>[2x]MWELTILHTNDVHSRLEQTSEDSSKCVNASRCMGGVARLFTKVQQI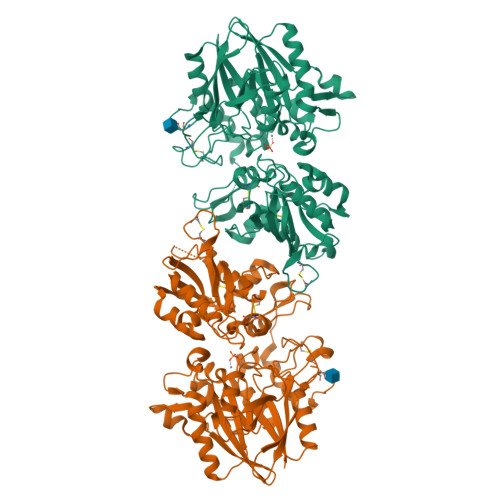RRAEPNVLLLDAGDQYQGTIWFTVYKGAEVAHFMNALRYDAMALGNHEFDNGVEGLIEPLLKEAKFPILSANIKAKGPLASQISGLYLPYKVLPVGDEVVGIVGYTSKETPFLSNPGTNLVFEDEITALQPEVDKLKTLNVNKIIALGHSGFEMDKLIAQKVRGVDVVVGGHSNTFLYTGNPPSKEVPAGKYPFIVTSDDGRKVPVVQAYAFGKYLGYLKIEFDERGNVISSHGNPILLNSSIPEDPSIKADINKWRIKLDNYSTQELGKTIVYLDGSSQSCRFRECNMGNLICDAMINNNLRHTDEMFWNHVSMCILNGGGIRSPIDERNNGTITWENLAAVLPFGGTFDLVQLKGSTLKKAFEHSVHRYGQSTGEFLQVGGIHVVYDLSRKPGDRVVKLDVLCTKCRVPSYDPLKMDEVYKVILPNFLANGGDGFQMIKDELLRHDSGDQDINVVSTYISKMKVIYPAVEGRIKFSHHHHHH>[2x]MDTIVKKTRTRLSPEKRKQQLLDFALDVFARRGIGRAGHADIAEMANVSVATVFNYFPTREALVEEVLLQVENRFSL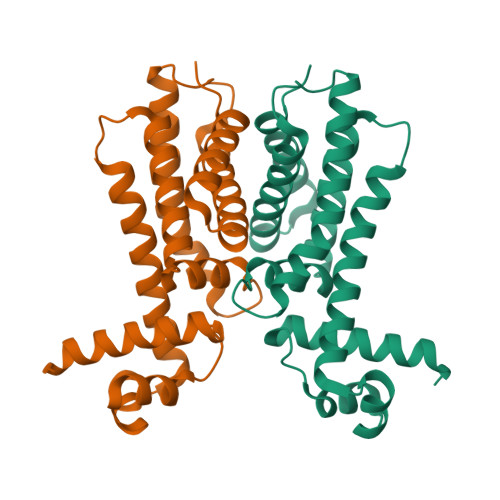LLSECLDEQDKTLHARLRGISHTLIDAVIEQQDWLKVWFEWSTSVRDDIWPQFISGNKKSLKRIAAAFEQGKENNEIDSDNSSDDLAHLLHGLCYILYLQSNLHPDQDRMREQAERYINTLYPAK(2S,3S)-2,3-dihydroxy-3-(1H-imidazol-5-yl)propyl 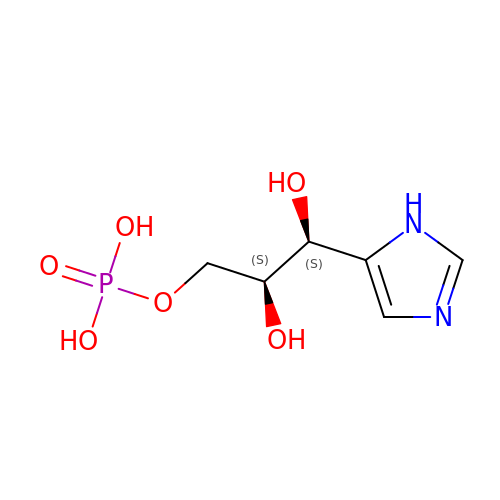dihydrogen phosphate | C6 H11 N2 O6 P | HFYBTHCYPKEDQQ-WDSKDSINSA-N>GSNKPPEFSFEKARVRKDSSEKKLITDALNKN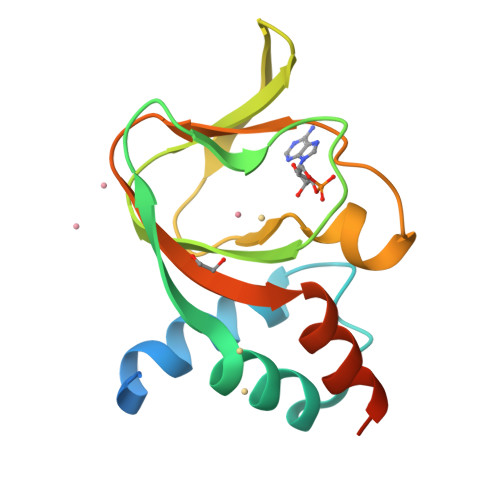QFLKRLDPQQIKDMVECMYGRNYQQGSYIIKQGEPGNHIFVLAEGRLEVFQGEKLLSSIPMWTTFGELAILYNCTRTASVKAITNVKTWALDREVFQNIMRRTAQARDEQY[2x]>[2x]GMATNSSTEQSLTKKVWNLATTLAGQGIGFTDYITQLTYLLFLKMDAENVEMFGEESAIPTGYQWADLIAFDGLDLVKQYEET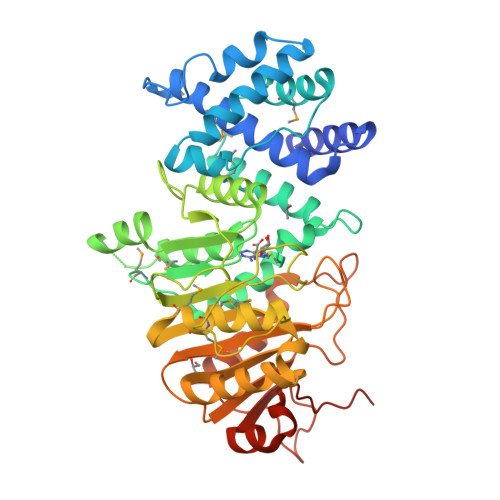LKLLSELDNLIGTIYTKAQNKIDKPVYLKKVITMIDEEQWLIMDGDVKGAIYESILEKNGQDKKSGAGQYFTPRPLIQAMVDCINPQMGETVCDPACGTGGFLLTAYDYMKGQSASKEKRDFLRDKALHGVDNTPLVVTLASMNLYLHGIGTDRSPIVCEDSLEKEPSTLVDVILANPPFGTRPAGSVDINRPDFYVETKNNQLNFLQHMMLMLKTGGRAAVVLPDNVLFEAGAGETIRKRLLQDFNLHTILRLPTGIFYAQGVKANVLFFSKGQPTKEIWFYDYRTDIKHTLATNKLERHHLDDFVSCYNNRVEIYDAENNPQGRWRKYPVDEIIARDKTSLDITWIKPGGEVDDRSLAEL PorL and PorM (GldL and GldM) are IM proteins that interact via their trans-membrane segments. PorM (or GldM) is therefore a central structural component of the T9SS and an interesting target for structure and function studies. Here, we present the atomic structures of the periplasmic domains of both PorM and GldM, that exhibit 22% amino-acid identity, and provide information regarding the contribution of each domain for interaction with PorK and PorN. Finally, we suggest that due to the structural similarity between PorM and GldM, both classical T9SS and Gld T9SS membrane core complexes might assemble and function in similar ways.

Full-length PorMp resisted all attempted crystallization assays. Phasing was performed using SeMet-substituted PorMp224. Domains D2 and D3 could be traced fairly easily, but domain D4 was only partially constructed due to poor electron density map. The D4 domain was easily traced in the electron density map because it was stabilized by nb130 binding, and it was introduced into the PorMp224 structure, generating a complete model. The resulting PorMp224 structure exhibits three domains that resemble GldMp domains D2–D4. Interestingly, PorMp domains D2 and D3 possess a domain-swapping motif identical to that of GldMp. Domains D3 and D4 of PorMp224 and PorMp315 share the same straight topology as those of GldM, whereas domain D2 is bent with respect to D3–D4 at an angle of ~45° because of the convolution of two rotations and a sliding of D3 monomers. The most striking difference observed between GldMp and PorMp is their overall topology, which results from the PorMp kink between D2 and D3. This kink is the result of two rotations around a vertical axis and around a horizontal axis, as in a cardan mount. Of note, the PorMp D2–D3 bending movement can occur in the left or the right direction, leading to two non-superimposable structures.

>SVDVGDYRVNSITAQVIPQSQIVMSGDTYKANIVLSSVDTTQRPDVFVNGKLLSPENMGLFTATAGAPGTYPVKGYIEMMGNDGVKIRRDFESEYFVTEPMASVAPTMMNVLYAGIDNPINIAVPGVAQQNVSATINNGTLTRRGNLWIARPTKVGSEAIISVTAQSGGRTIQMAKTTLRVRALPDPLPYIEYKDVQGNTKRFKGGRLGKREILAAGGIKAALDDDLLEVNYTVVKFQLVFYDSMGNSIPEVSDGASFSERQKRQIQNLGKGKRFYVTEVIARGPDGIERKIPAIEVIVN[2x]>GFNGGFG[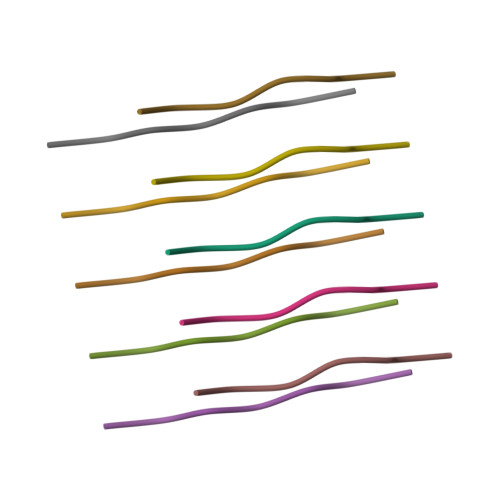2x]2-azanyl-2-[[4-[2-[3-[[2-[(1S)-1-oxidanylethyl]imidazol-1-yl]methyl]-1,2-oxazol-5-yl]ethynyl]phenoxy]methyl]propane-1,3-diol 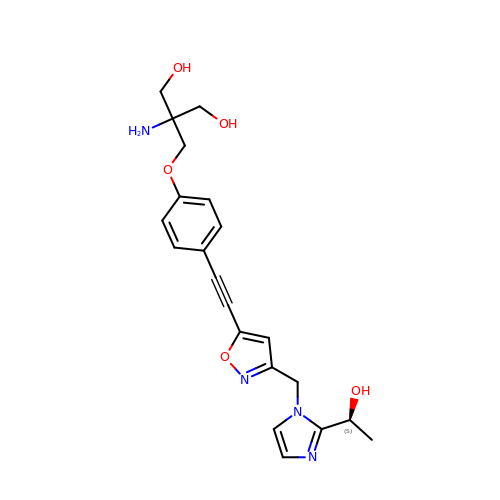| C21 H24 N4 O5 | DKGUWMFQYQOPSO-HNNXBMFYSA-N> QIGWRREGIKYRRNELFLDVLESVNLLMSPQGQVLSAHVSGRVVMKSYLSGMPECKFGMNDKIVIEKQGKGTADETSKSGKQSIAIDDCTFHQCVRLSKFDSERSISFIPPDGEFELMRYRTTKDIILPFRVIPLVREVGRTKLEVKVVIKSNFKPSLLAQKIEVRIPTPLNTSGVQVICMKGKAKYKASENAIVWKIKRMAGMKESQISAEIELLPTNDKKKWARPPISMNFEVPFAPSGLKVRYLKVFEPKLNYSDHDVIKWVRYIGRSGIYETRC;> DYMPMSPK

Clathrin-mediated endocytosis (CME) is a major regulator of RTKs involving the heterotetrameric AP2 complex composed of large α and β2, medium μ2, and small σ2 subunits. AP2 binds to transmembrane cargo proteins that contain specific motifs such as YxxΦ (Y denotes Tyr; x, any amino acid; and Φ, bulky hydrophobic residue) serving as μ2 binding sites. In this study, we discovered AP2 is also an IRS-1-associated protein. IRS-1 binds with AP2 to prevent IGF-IR recruitment into clathrin-coated structures and thus enhance surface retention of activated IGF-IR.

We also analyzed the crystal structures of μ2 C-terminal subdomain (C-μ2) bound to IRS-1 YxxΦ motifs. Importantly, the side chains of Tyr and Met residues of IRS-1 YxxΦ motifs are inserted into the binding pockets of μ2, which are shared by the AP2 cargo proteins. Collectively, these results indicate that IRS-1 is recognized by the AP2 complex via the μ2 subunit in the very similar manner to conventional endocytic cargos. Using IRS-1 truncated mutants, we mapped the central region (amino acid residues 543–865) which is necessary for the binding to AP2. This region is almost identical to that for the clathrin adaptor AP1 complex found in our previous study, which binds to YxxΦ motifs of IRS-1 including Tyr 608, Tyr 628, and Tyr 658 via its μ1 subunit. Indeed, the Ala mutation of all these Tyr residues in IRS-1, but not a single substitution, completely abolished the binding to μ2 in vitro (IRS-1 3YA mutant). The Tyr residues of the YxxΦ motifs of IRS-1 (Tyr608, 628, and 658) critical for the binding to AP2 are part of phosphorylation sites among multiple Tyr residues in the C-terminus of IRS-1 that mediate the interaction of IRS-1 with PI3K and subsequent activation of PI3K. In addition, AP2 would preferentially bind non-phosphorylated IRS-1 since AP2 cannot recognize phosphorylated YxxΦ sequence due to its limited capacity. Our results indicate that IRS-1 inhibits the recruitment of IGF-IR to CCPs through YxxΦ motifs in IRS-1.>ATYMLPSLHDI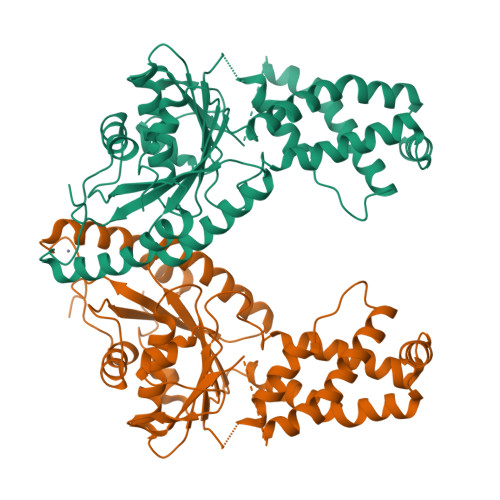LDQHTYKWIFFGGKGGVGKTTTSSSFSVLMAETRPNEKFLLLSTDPAHNISDAFDQKFGKAPTQVSGIPNLYAMEVDASNEMKSAVEAVQKETGSAADNDAESKSEGDMFGGLNDLITCASSFIKDGTFPGMDEMWSFINLIKLIDTNEYSTVIFDTAPTGHTLRFLELPETVNKVLEIFTRLKDNMGGMLSMVMQTMGLSQNDIFGLIDKTYPKIDVVKRISAEFRDPSLCTFVGVCIPEFLSLYETERLVQRLAVLDMDCHAIVINFVLDANAATPCSMCRSRARMQNKYIDQINELYDDFNIVLSPLRHDEVRGIANLRDYAETLIKPYRFCWSAN[2x]>[2x]GGTDINKLIEEGKKHYLPKTYTFDNGKIIIKAGDKVEESKIQKLYWASKEVKSQFHRIIGNDKPLEVGNADDILTIVIYNNPEEYKLNKTLYGYSVDNGGIYIEGIGTFFTYERTPQESIYSLEELFRHEFTHYLQGRYLIPG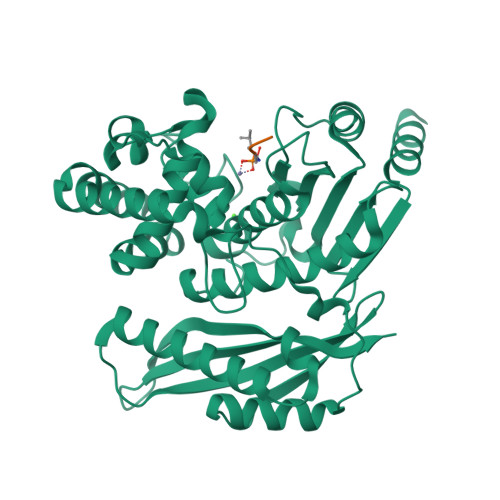LFNKGDFYKGNNGRITWFEEGSAEFFAGSTRTSVLPRKSMVGGLSKNPKERFNADKLLHSKYSDGWDFYKYGYAFSDYMYNNNKKLFSDLVSTMKNNDVKGYEALIEESSKDSKINKDYEYHMENLVNNYDNYTIPLVSDDYMKQYDNKSLHEIKSDIEKAMDVKNSQITKESSQYFDTYNLKATYTLSSNKGEISNWNYMNNKINEALNKLDNLSWGGYKTVTAYFSNPRLNSNNEVVYDIVFHGLLSHN>[18x]MTTTITIPNSYPIFTPNQVLTNKDLNRVVTYLDEQNRLTRVYLIGMGIVAGMEVSSIYQPGDVNIVVAPGCGITSEGYIISLAETKLTHYQSGVSVPSALFAPSEEQTAASTDQLVELFEQEGNNRLALKNLPDENAFARFLADQTLVVVYELQDQQRDSCLLDCDDTGKDRNFRLRYFLLPRSVPEKLSAEALLQQGFSREPLPQQWRDFSINDIFQAQSSFFQNFFPQVRRFGYTLETPPVIRLSNIVDYDAFLKGYQQVCLQAIDEIDRTFPNLFRLFSPFFSSFNPAPSDFTGLKTLLNQRLSDIVSGSSAENRRSPISQIEAQYALQYFYDYLSQLVSAFRELAESAFDLMDDATPDTRRFPKFLMLGLVPLPNQKPEVYALNSPYRSNFSQSPIYNGNQLRVKQVRFLYDRLVRLCAADSFYLLPFYDTPLKITPSKDRAATLSQQAIPYYLNYPQLYQYWSYDTYRKGRSQSHPAYFYPNNANITPNSDLLHRLDDYSFYRIEGHIGEANATALQRILDYQQRYNLAFDVITLKIGNLQSFQDINISGQFDDLNADFGRIKDTFAKLWQRYEESWSRNVFLYTLKRVFFDKTSLAEIKSDQLFNPIVARASVKEAYEFVKESGDSYRLYLRNAAGIRIARFETVINFSGLSGDSLTQEQERIIGDLLACLPLGKITYGVEPESANNPLSYYLRFSLADELDLPANRGTADISFISLNFFTVNFEGNSPIINQPEFQDFETLYSLLRDVPESSIRVNRLELRMGDRLAADTLNYFELKGLMTAYQQRLAQIMELQLFHKFAQNNPGMEHLGGVPKGGTFVLVYVDGRELVRNLLSADRDPTYQARTEVIKKYASLPPGSPQELATSRELLNREDIVVGDFCLPYRFSSKTPTVSYVLTQPRPIVLLDRTTFCAGDETRYEFILDPTGGTLKGEGSFFADGKYYFQPSRITDDITSETAITFTYVVESSYDTLSVTVYPLPDASFQIKTNFCSNENPVTLRATQPGGNFRAFDSETDISASVINNQEFNPSAVNLGGATEKVITLVYTITSDQGCTNELSRDITIFAVPNATFQVGQGKTRFCSNDEPVDLIARVPGGTFQVRDGAEDISADVINRLTTPPQFDPSAVNLGVAREKVITLEYSISNQGCSNKFTQELRIFAVPNANFRLSTGNRDTFTNNDPPVGLIATQLGGTFQAFDGEEDITADVISPTTPPQFNPSAVNLGDEEEKVITLRYTISNQGCSNNTERRVTIVPPPEVPVRDVEDTSNPDSGDAPTENPIPHPEVRAVNLLAISNNEVINSTNLDGDRTFNLSDFNPNNQYTFEAMTVPEKVNSVIFTYTKPNGSRQALTANTAPYRMPDDWQPSIGIHEIQAQAIREVNGDRLEGATIKVIIRVIDADTDTSPSRSTNPDNLFTRIQNLFPLNRGEIITKIKLPQLLAMSTAIFMLIVGWTYSSSKQVGSTPPSVIKPR;>[6x]MPEYLSISKQKPDFPPYL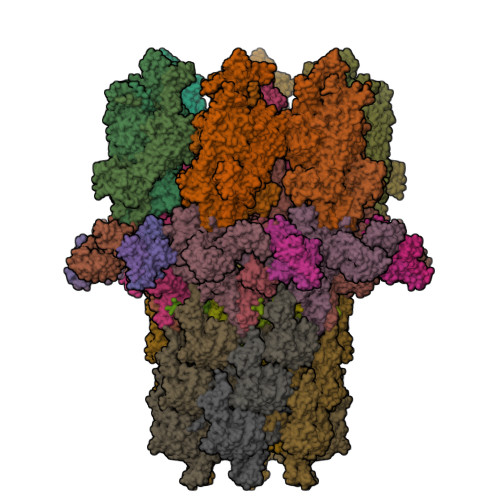NFQTLRDIGITHLQALSGKIWTDYNLHDPGVTILEVLCYAITDLGYRNNLDIADLLALNPQDGNSRENNFFTPDAVLTCNPVTELDVRKRLIDIPGVRNAWLQKVTSYEPNIYVNFSDKRLQYNPPTAESKTLNPRGLYTVRLDLDQDYRKNACGQIDRSWGDTLDEVKQVLCDSRNLCEDFADIVILGEEEIGICADIQLETNADAEDVLVNIYVRIQQFLSPRLKFYTLQELLDKGKSPAEIFAGRPSVFDGENRLYKSHGFIDTDELEALTLPTILHTSDLYQEILQVPGVSAIKKLSIANYINGLRQTQGHPWYLQLTDQYRPVLGVKTSKINFFKSELPIGVDEEEVERRYYEQQAAYIKTIRDRDELDIPVPKGSYYDLADHYSIHHDFPTTYGISEDGLPPTVPALRKAQALQLKAYLVFFDQLLASYLAQLSHIRDLFSWEVDVTQPQQNDYATRLQEKQRTYFTQKLDFPEIEKIIPDNYLDVLDEAPETYRDRRNRFLDHLLARFSESFSDYVLLNYQMFATRNNKATQETEIIHDKAQFLQDYPTLSRDRFRAYNYYDCHAVWDTDNVAGFKKRVLRLLGIDDVRRRHLSHYRVDKDSRNLFLSIDFSSDDLTLTSKQRYATTEQAQADQDKLLLFALHPNFYKRLSYKYYYHYSWEILDTQNQSIVRSDRFFPSTKERAAALEPLLQSLLTQLSQLDDTALQNLVITQPTDEDLYSFRLQIPLNSGVITFTGVQRYFSRTEAVDAGVISLRLIQDVQNYRNITLGQDQGTTPQKFTYYGYGLVDHQGSLLSEYTHHFPTELERELSLQRWLTHIQANQNQYKFAIETITNGYVFVINDITNSQTLLRGISSYATEYLAWQAASEFAENLRYLNRYLSPAKDHTGQTYSLGITDKTGKLLAVTTTESDRLLTFQRLNALEPFLVIEAATTPTSGYRYRLVDRQETTILQSIQIYGDETTARDRFYQDVLGTLFETGVINPTTTNKEFGFRILSRPRDTNSVAAIHTQTYTSEAERDAAIEHLLLLVRTARLRISTNSLDSLAYISQIYNPDNQLILQGTQRYTSEDIAWEQGNTLMELAQDEENFRLIDSDDGVYGWELTNEGKDEIFAAQYYNSREERTAAIAEIQKYSNDEGFHLLEHILLRPRTKLPDLTAGDGFLPILVTPEDVNTEPDDPYLLARTDPYSFWVTIVLPYWPQRFRDIPFRRFVERTLRLEAPAHIALKIAWVNVRQMRDFELAYRHWLEQLALESCENAACDLTGTLNRLLKILPQLRNVYPKATLHDCEESSADNNPAILNQTALGTAND;>[18x]MNLRKRNELKSLFKNKSRLSETYFVELIDSTLNKRDDRFHGIWKPGQTYQKGDVVYYNHSLWEMQSENEICAKEEQTPGISTDWKSLLKELEQKVDKLQHELETLHQEFTEYQKQMEIRLQLLARFIPILFIGLGIMFFWLLGQSTVHILAGTT;>[6x]MSNNRDLPKNPLIRDGVSQRQRQVSALSPASIGVDERDLADFLVLVYRLSAKVMYYRAENQPWSPSDADGNWQNFFEGNTPIQIALISKVSPQVVKDIYSQKLAAFLAERTVTSLSEVLSIWKTEILTKIQQWYLGIEAYTPLKSVIKGLVKTNLTEPLMRMQSFELGCGNVDEEFYRGFSGVFGLTIDAPLRSDRTPLMGTVKDARTELDTVFQVLLQTYRQIIQQAPNYLKASLSDRQDHQPFLSLYFAFLEVLQPARDDLNRLTQRHLDFFYRQVLLLPDRPAQADQVHLLFELAKSQREYKLTAGTSFKAGKDATGVDLFYQLDAETVIHKAQIASLKGLFLDSQERKTAAVPQNLTGLYASPVANSVDGKGGAFPQEQIVKTWLPFGNEQRDHARLGVAIASDVLLLQEGRRVVEFKLSLGGFFPRLPDNQLHQAFVVYLSGEKAWIPAPILPVGQLATNGQEQTRWDGSNLYLVVELAADVAPILPYRPDAPIPYDPKELNLPLQLERPIPVARLELNHQLLVNERSPYHYFRDAQILDITVQTRVDEVRNLVVQNDVSVLNPARPFEPFGFQPQDKANLYIGSQEVLQKRLIALTISLELATPKPNNWIEFYAGYDIPANFQPGKVKIQGLRQKTWYPTTANVTANLLDTPEISLTSKLANLKLDSFDQSAPVEMFTPQTKTGFLRLQLSGNFLHEQYPRVLAKQVLAAATNQTVVVSSNQKRQAVIGAYYRRPDKSIFAATTYYVNLDDEPIIPNEPYLPVVRSLSLKYTAQAGMSDCILFHLHPFGGFAKVNLAVNPPLLPYFNQEGELFIGLQNLDPPTALPLLFQVAEETADISLRRQEEYKLQWYYLKDNAWESLGDRIVNDASNGLVTSGIINLGIPADISRNQTTILDPNFHWLKVTIPARSRTVCEIIGVHTQAARVTFKDAGNDPNHLGSPLAGGTISKLAVPQPEVKKIAQPYTSFGGRVKEQPENFYIRISERLRHKGRAVAIFDYERLVLEKFPQIYKVRCINHGQFDDAQEQLYELAPGSVTLAVIPDLSQRSTTNDLEPKVNINLLQEIEKYLASVSSPWAMIKVVNPQYERIQVDFQVKLKAPYSSNFGYYRRELQQAIVGFLTPWTVDSGADINFGGKVYRSSILKFVEEQYYVDYVVNFKMNLNNQQDIREAIAITPRSVITSVSPKTSNQDHMIEEFIEQAIVFNNQKLESGVLGYESLNDLELGE;>[6x]MDDESNAYLGTGWGFPPTFEKKARSVRLVSAEDDIRESLQILLSTNLGERVMQPNYGCNLQDLLFESLSPTVASNIKELVRTAILYYEPRIRLNKLDIQQGISDRQNPSAVNEADAQGLIQIIVDCTIISTNSRFNFVYPFYLQEGSGN;>[3x]MNDRIIPRNSLYDVATFKLLSDGKDITNDYTVLSITVNQIVNRVPTARIILRDGAAADETFAASEGADLVPGQEVEIAAGYDGSDQKIFQGLIVKHALKVTANGDSMLMLDCRGLATKLTVGRHNRYFVDTKDSDAIAEIIAQHSLSADVAATQVQHPEIVQYYATDWDFILSRAEMNGQIVVAQDEKIKVKAPNTSGAPQITLTYGVNLLELEAAMDARHQYQAVKATSWNYADQALVEAEASEPTVNNQGNLSGRQLAQVIDLSALELRHSGLVAEPELKAWADAQLLKSRLAKIQGRVKTKGYPDAKVDVLIQLAGVGDRFNGLAYVSGIRHEIVGGAWDTHIQMGLPPQWFYQEVDIIDKPAAGLLPGVNGLQIGVVVQLQDDPNGEDRILVKVPIIDAQAEGIWARIATLDAGNNRGSFFRPEVGDEVILGFLNDDPRDPVVLGMLNSSAKPAPLRATAENHRKGFFTRSQMQLTFDDDKKIITLQTPGGNKVTISDEDKGITLTDQNGNTFAMSDRGIAMNSPKDITLEATGKLTLKATQDVSIEGLNVNIAANAQFKAQGNAGAEVSSSAIAVLKGSLVMIN;>[6x]MALTKVKLLAYQDKRFENKLGEFELPINPEQFSQSFKVEYNREQAQGSQRNDPEFKFTKPEELKLDFTFDGTGVVPVNNGKPGEFHQDVADQVRVFLDLVYSMNSETHKPNFLRLIWGDFSFGEKNGFDCLLTDLQINYTLFDQTGKPLRAKLSTTFTSYVEQNRRVREEGKQSPDVTHQRKVKAGDTLPLMTHRIYGDPAYYLQIAKVNGLINFRKLATNTDLRFPPLEKTQS;>[3x]MPLEIRELVIKASVNEGGQNQGTGGAGDQSAIIAACVEQVLAILQEKSER;>MIRTYPPVSFFFEVVFQGENLDKDVVETRFQSVTGLSVDMQTETLKEGGENRFEHILPVRTKYDPLVLKRGLVNDSQMVKWCMDAILNFDIRPMNLLVRLLHIERSDPNQPPEAIATGGSSTIAPLMTWKVINAWPKKWSVSEFNAEQNSIAVESLELNYSYFETLK[6x];>MAEYPLPKFHFQVDWGGSRLGFTEVSGLDVETEVIEYREGNLPQYHKLKMPGMQKFSNITMKRGTFQGDNDFYKWWNTVALNTIERRDLTISLLNEKHEPVVVWKVNRAWPTKVQSTDLKGDGNEVAIESIEVAHEGLTIQNG[6x];>MPSTYKTPGVYIEEISKFPPSIAQVETAIPAFIGYTQIAKVGVENFHTDADNLILRPVRITSLLEYEQFFGKAINETTIQVVIQDTTDSRGNLTERKASARITSPSPHNLYYSMQAYFANGGGPCYIVSVGPMSNTGTIQLEALQNGLAEVAKEDEVTLLVFPESQSLSDENYAALMSAALEQCANLQDRFTVMDLKLPATRPIPANAIVGASNAFRDLSLPQDNLKYGACYAPDIETIFNYFYQEDAVTIFRSVNGGAEEQDTLTMAGYNPANGGDGIQYALIESAIDQLPLILPPSPLVVGQYARTDNTRGVWKAPANVALSSVIKPVLKITNEQQNNLNVHPTGKSINAIRAFTGKGTLIWGARTLAGNDNEWRYVSVRRFFNMAEESIKKGSEPFVFEPNDANTWTKVKAMIENFLTLQWRAGALAGAKPEQAFYVKIGLNETMTALDILEGRMIVEIGMAVVRPAEFIILKFSHKMQES[18x]>MSLNRFTKTSQGRSWNTGNGSPDAICFAVDKPGIVVVGFAVYGGGGIHEYELEVLVDDSEHAGDSTHSHRWTSLELVKGTYTTDDSPSDIAEIRLDKVVPLKENVKYAVRLRNYGSRTANGDGGMTTVQCPDGVTFTFSTCSLSSNGTNQTRGQIP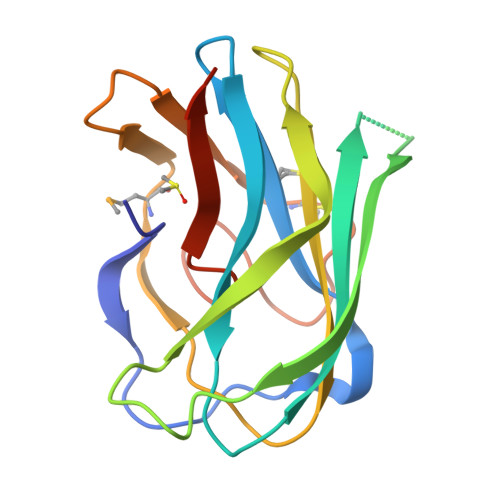QILYYRSEEGHHHHHH[2x]>[2x]MPRGLELLIAQTILQGFDAQYGRFLEVTSGAQQRFEQADWHAVQQAMKNRIHLYDHHVGLVVEQLRCITNGQSTDAEFLLRVKEHYTRLLPDYPRFEIAESFFNSVYCRLFDHRSLTPERLFIFSSQPERRFRTIPRPLAKDFHPDHGWESLLMRVISDLPLRLHWQNKSRDIHYIIRHLTETLGPENLSKSHLQVANELFYRNKAAWLVGKLITPSGTLPFLLPIHQTDDGELFIDTCLTTTAEASIVFGFARSYFMVYAPLPAALVEWLREILPGKTTAELYMAIGCQKHAKTESYREYLVYLQGCNEQFIEAPGIRGMVMLVFTLPGFDRVFKVIKDKFAPQKEMSAAHVRACYQLVKEHDRVGRMADTQEFENFVLEKRHISPALMELLLQEAAEKITDLGEQIVIRHLYIERRMV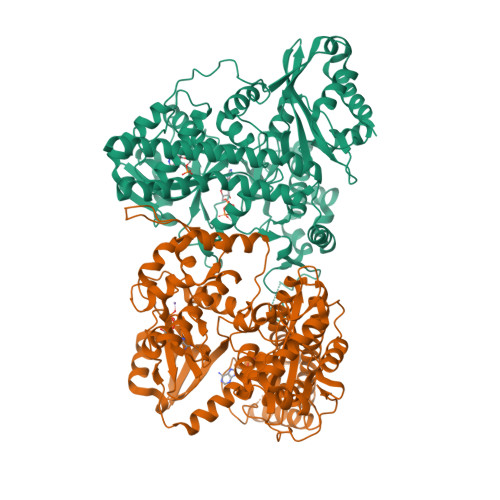PLNIWLEQVEGQQLRDAIEEYGNAIRQLAAANIFPGDMLFKNFGVTRHGRVVFYDYDEICYMTEVNFRDIPPPRYPEDELASEPWYSVSPGDVFPEEFRHWLCADPRIGPLFEEMHADLFRADYWRALQNRIREGHVEDVYAYRRRQRFSVRYGEMLF>[6x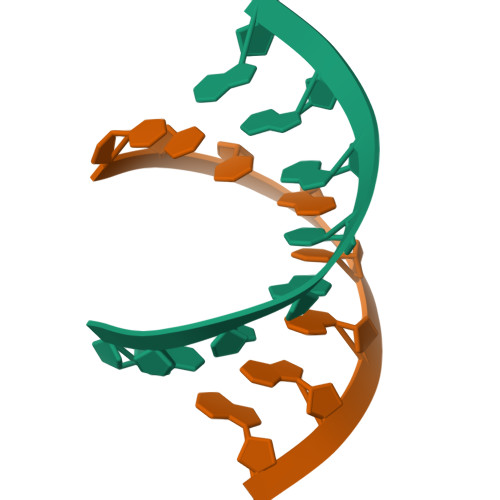]CCCIUGGG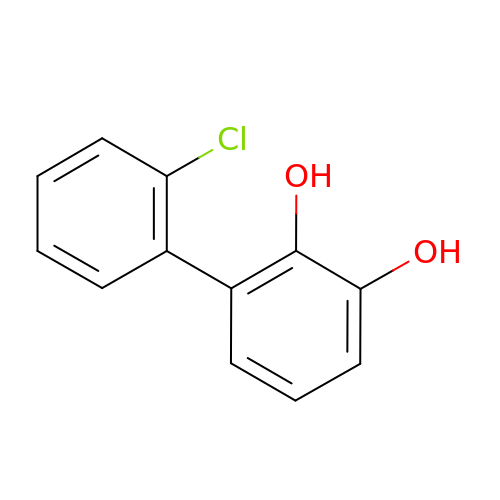2'-CHLORO-BIPHENYL-2,3-DIOL | C12 H9 Cl O2 | SNGROCQMAKYWRE-UHFFFAOYSA-N The Hermes DNA transposon is a member of the eukaryotic hAT superfamily, and its transposase forms a ring-shaped tetramer of dimers. The Hermes transposase is composed of 612 amino acids and is organized in four domains. Architecturally, the Hermes transposase is unusual as it spontaneously forms a ring-shaped tetramer of dimers. All hAT transposases are predicted to contain an N-terminal BED zinc-finger domain organized around a conserved CCHH or CCHC motif that coordinates Zn2+13, but no structural information is available for Hermes as the constructs used in previous structural work lacked the first 78 amino acids.

The complex crystallized in space group P6522 with a crystallographic twofold axis perpendicular to the oligonucleotide that intersected it at its central base pair. Thus, the asymmetric unit contained one BED domain and one DNA strand of the duplex. Each BED domain contains at its C-terminal a CCHC zinc-finger involving residues C51, C54, H71, and C73 that coordinate a bound Zn2+ ion. The two BED domains bound to the imperfect palindrome do not contact each other, but each C-terminal α-helix between T65 and R70 (α3) is deeply inserted into the major groove. Key to binding the imperfect palindrome is the ability of the N67/R70 pair of the BED domain to assume alternate conformations. In the other half (BED2, shown in green), the position that was occupied by A18 is now replaced by G20, which is less competent to interact with N67. We observe that N67 is completely displaced, no longer facing the DNA but instead interacting with K59 and the phosphate of G19, with R70 now in its place to interact with G19. Thus, the structure shows that the single BED domain of the Hermes monomer is able to form specific interactions with two related but distinct DNA motifs. Therefore, only simultaneous double interaction events were observed consistent with cooperative binding. As the crystal structure of the BED/DNA complex showed no evidence of protein-protein contacts, it appears therefore, that cooperativity is the result of DNA deformation.

> MQKMDNLEVKAKINQGLYKITPRHKGTSFIWNVLADIQKEDDTLVEGWVFCRKCEKVLKYTTRQTSNLCRHKCCASLK3-[[6-bromanyl-2-[3-(dimethylamino)propyl-methyl-amino]quinazolin-4-yl]-methyl-amino]propanenitrile | C18 H25 Br 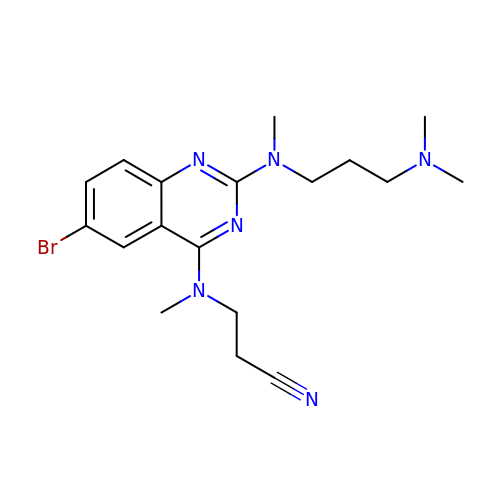N6 | YQHWFKUKSRPCIG-UHFFFAOYSA-N> GSDELYRQSLEIISRYLREQATGAKDTKPMGRSGATSRKALETLRRVGDGVQRNHETAFQGMLRKLDIKNEDDVKSLSRVMIHVFSDGVTNWGRIVTLISFGAFVAKHLKTINQESCIEPLAESITDVLVRTKRDWLVKQRGWDGFVEF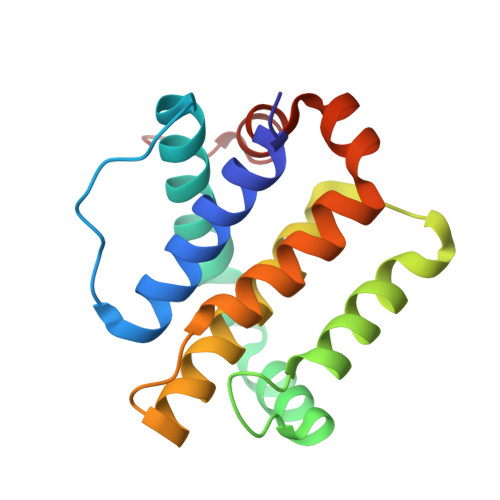FHVEDL4-[(3-aminophenyl)amino]pyrido[2,3-d]pyrimidin-5(6H)-one | C13 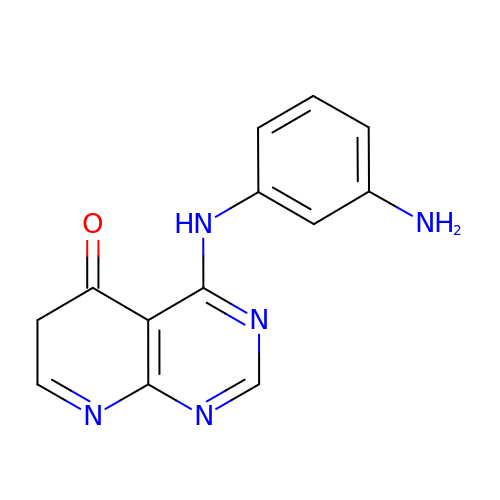H11 N5 O | PWIXWXGXVKPITN-UHFFFAOYSA-N> MDDEDNKCDCPPPGLPLWMGTFADLMSLLMCFFVLLLSFSEMDVLKFKQIAGSMKFAFGVQNQLEVKDIPKGTSIIAQEFRPGRPEPTPIDVIMQQTMDITQQTLEFHEGESERAGGTKRDEGKLTGGQSPETSTQNNESAEADMQQQQSKEMSQEMETLMESIKKALEREIEQGAIEVENLGQQIVIRMREKGAFPEGSAFLQPKFRPLVRQIAELVKDVPGIVRVSGHTDNRPLDSELY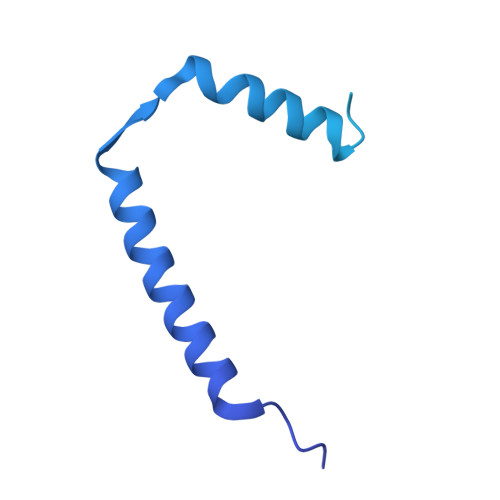RSNWDLSSQRAVSVAQEMEKVRGFSHQRLRVRGMADTEPLLPNDSDENRALNRRVEISIMQGEPLYSEEVPVIQ> MAGSPELVVLDPPWDKELAAGTESQALVSATPREDFRVRCTSKRAVTEMLQLCGRFVQKLGDALPEEIREPALRDAQWTFESAVQENISINGQAWQEASDNCFMDSDIKVLEDQFDEIIVDIATKRKQYPRKILECVIKTIKAKQE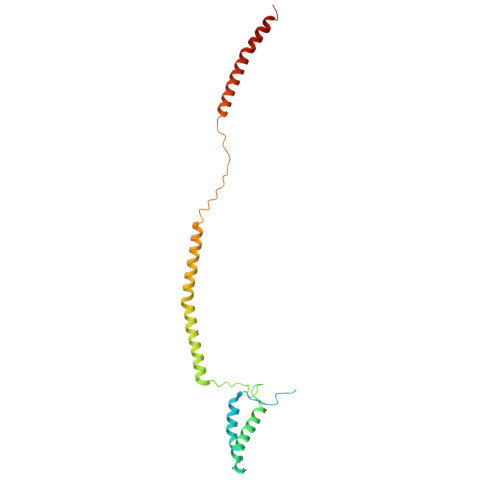ILKQYHPVVHPLDLKYDPDPAPHMENLKCRGETVAKEISEAMKSLPALIEQGEGFSQVLR>GSGASQFFKDNCNRTTASLVEGVELTKYISDINNNTDGMYVVSSTGGVWRISRAKDYPDNVMTAEMRKIAMAAVLSGMRVNMCASPASSPNVIWAIELEAEGS[2x];>[3x]GASQFFKDNCNRTTASLVEGVELTKYISDINNNTDGMYVVSSTGGVWRISRAKDYPDNVMTAEMRKIAMAAVLSGMRVNMCASPASSPN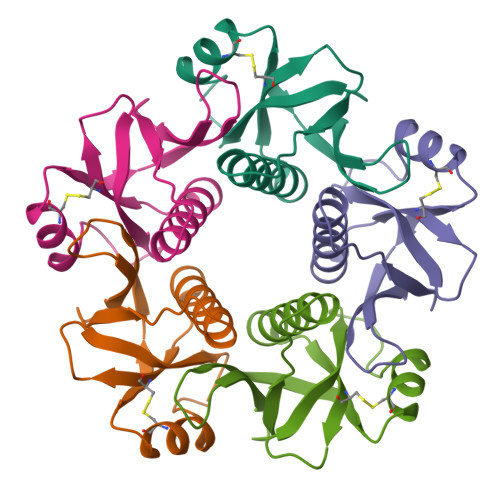VIWAIELEAEGSGS D-VINYLGLYCINE | C4 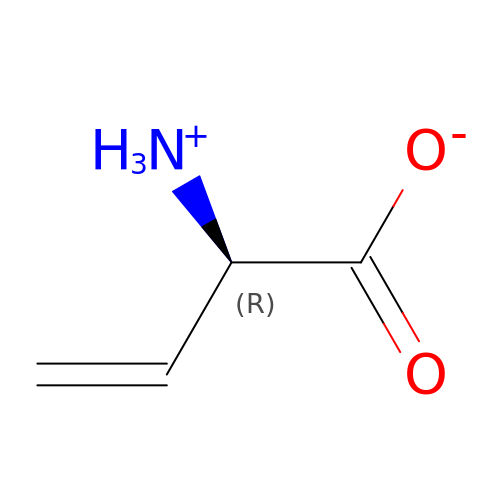H7 N O2 | RQVLGLPAZTUBKX-GSVOUGTGSA-N> STRDYEIQRERIELGRCIGEGQFGDVHQGIYMSPENPAMAVAIKTCKNCTSDSVREKFLQEALTMRQFDHPHIVKLIGVITENPVWIIMELCTLGELRSFLQVRKFSLDLASLILYAYQLSTALAYLESKRFVHRDIAARNVLVSATDCVKLGDFGLSRYMEDSTYYKASKGKLPIKWMAPESINFRRFTSASDVWMFGVCMWEILMHGVKPFQGVKNNDVIGRIENGERLPMPPNCPPTLYSLMTKCWAYDPSRRPRFTELKAQLSTILEEEKLQ

Focal Adhesion Kinase (FAK) is a non-receptor tyrosine kinase that regulates signals involved in cell proliferation, migration and survival. FAK activation is initiated by breaking an intramolecular autoinhibitory interaction between the N-terminal FERM (4.1, ezrin, radixin, moesin homology) and kinase domains. All compounds exhibit a common 5-chloro-2-ortho-methoxyanilino-4-anilinopyrimidine core structure, which binds in a nearly identical manner to the hinge region of the FAK kinase.

TAE226 is a potent inhibitor of FAK (IC50 = 5.5 nM) and also inhibits insulin receptor (InsR) and insulin-like growth factor-I receptor (IGF-IR), albeit ∼10 fold less potently (IC50 = 44 nM for InsR and IC50 = 140 nM for IGF-IR). The methyl carbamoyl moiety in ortho position to the amine in the 4-aniline ring of TAE226 is located near the DFG motif of the activation loop of the FAK kinase. Its carbonyl group forms a hydrogen bond with the backbone nitrogen of Asp564 of the DFG motif. The side chain of Leu567, the residue immediately following the DFG sequence, makes hydrophobic contacts with the 4-aniline ring. Interestingly, the interactions involving Asp564 and Leu567 stabilize a short helix that includes the DFG motif. This conformation of the DFG motif, which is induced by these contacts with TAE226, is similar to the conformation induced by the bis-amino pyrimidine FAK inhibiter PF-562,271 and has to our knowledge only been observed in FAK. In order to adopt this helical turn the phi torsion angle of Asp564 is rotated by 113° compared to the active kinase domain. Together, the backbone rotations of Gly563 and Asp564 move the Cα of Asp564 by 3 Å closer to the N-lobe with its side chain closely approaching the N-lobe of the kinase. Interestingly, the FAK inhibitor TAE226 induces a DFG conformation in FAK that is distinct from that observed in Abl or other kinases. Our work demonstrates that TAE226 locks the activation loop of FAK into a helical conformation, which to date has only been observed in FAK and appears to require a glycine residue immediately preceding the DFG motif.>MTSEHRSASVTPAHIAMFSIAAHGHVNPSLEVIRELVARGHRVTYAIPPVFADKVAATGARPVLYHSTLPKPSNPEESWPEDQESAMGLFLNDAIQALPQLADAYADDIPDLVLHDITSYPARVLARRWGVPAVSLSPNLVAWKGYEEEVAEPMWREPRQTERGRAYYARFEAWLKENGITEHPDTFASHPPRSLVLIPKALQPHADRVDEDVYTFVGACQGDRAEEGGWQRPAGAEKVVLVSLGSAFTKQPAFYRECVRAFGNLPGWHLVLQIGRKVTPAELGELPPNVEVHQWVPQLD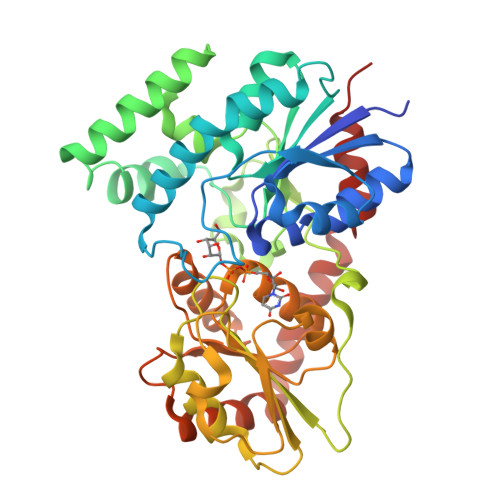ILTKASAFITHAGMGSTMEALSNAVPMIAVPQAVDQFGNADMLQGLGVARKLATEEATADLLRETALALVDDPEVARRLRRIQAEMAQEGGTRRAADLIEAELPARHG[2x]> EFLTFNVPSSPPSNSSAQLSDAPVGVSFEFFAFPGYWNDVPSTSTCLQNLKDLSGTWPPIRIGGTTQDRATYDASSSQQVT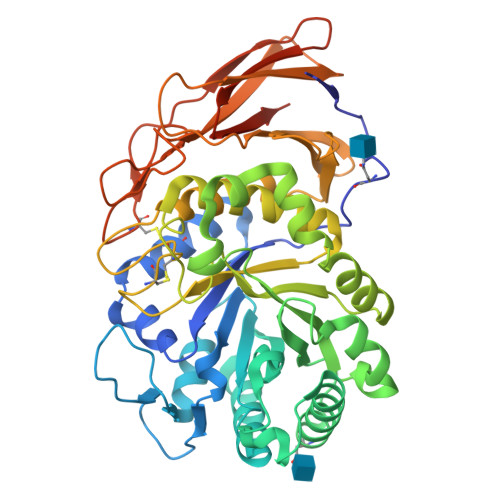YTVANAGDAPSTLTFGPSFMSLAGTYAGQVTIGFNRRLNNLANTVAAASKAVNEINSLHAIELGNEPNFFSGSDPIAQGSSWTASADYASEVTWQDAVCGNLSASNLISAGVFFGTSPMSIAGLTAVEGQANSYVRQYCSHNYPQSKSTANLANLMSHSGIASQIKPFAKEVAAALAKNKPHVFGETNSATQGGGGISPTYGAGLWLLDYVMQALIMGTETLYFHHGTIGNCQYCWWGKYSMGSPYFGAYFATMALAGANKIAPLDDQTTGYAAYAIYKDDKPIRVLLYNSDYYTSGSRPSQTFTLTGLSGSTVSAKRLTAAASTSRVDAGQSPTVAGQTFENGSCKIQGQSTVESATVSGGKATFTLQASEALLVTLENKLISEEDLQSAVDHHHHHH> NVLTVYSPYQSNLIRPILNEFEKQEHVKIEIKHGSTQVLLSNLHNEDFSERGDVFMGGVLSETIDHPEDFVPYQDTSVTQQLEDYRSNNKYVTSFLLMPTVIVVNSDLQGDIKIRGYQDLLQPILKGKIAYSN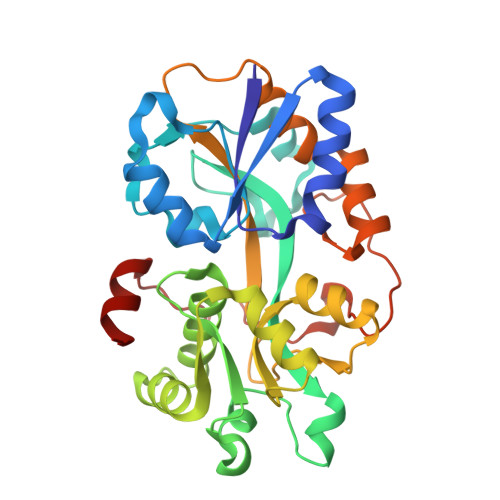PNTTTTGYQHMRAIYSMHHRVSDVHQFQNHAMQLSKTSKVIEDVAKGKYYAGLSYEQDARTWKNKGYPVSIVYPIEGTMLNVDGIALVKNAHPHPKRKKLVQYLTSRSVQQRLVAEFDAKSIRKDVSEQSDQSIENLKNIPLIPKSKLPDIPHHKFLEMIQ> MGHHHHHHAENLYFQGADPFESYNPEFFLYDIFLKFCLKYIDGEICHDLFLLLGKYNILPYDTSNDSIYACTNIKHLDFINPFGVAAGFDKNGVCIDSILKLGFSFIEIGTITPRGQTGNAKPRIFRDVESRSIINSFGFNNMGCDKVTENLILFRKRQEEDKLLSKHIVGVSIGKNKDTVNIVDDLKYCINKIGRYADYIAINVSSPNTPGLRDNQEAGKLKNIILSVKEEIDNLEKNNIMNDEFLWFNTTKKKPLVFVKLAPDLNQEQKKEIADVLLETNIDGMIISNTTTQINDIKSFENKKGGVSGAKLKDISTKFICEMYNYTNKQIPIIASGGIFSGLDALEKIEA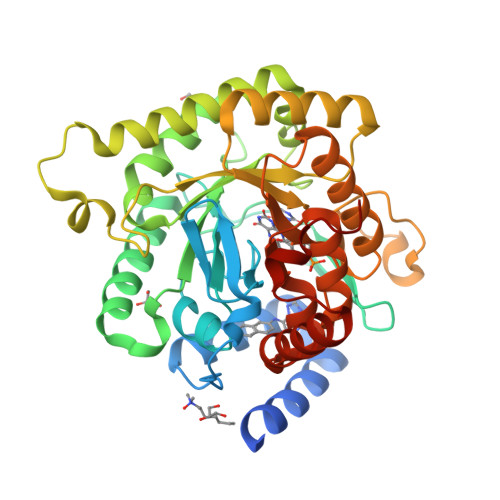GASVCQLYSCLVFNGMKSAVQIKRELNHLLYQRGYYNLKEAIGRKHSKS>[6x]MAPKRKASSTCKTPKRQCIPKPGCCP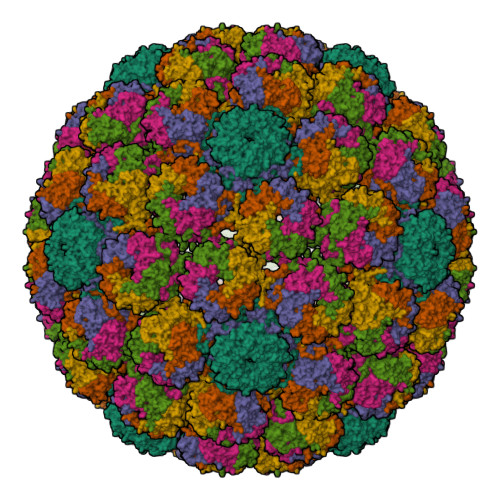NVASVPKLLVKGGVEVLSVVTGEDSITQIELYLNPRMGVNSPDLPTTSNWYTYTYDLQPKGSSPDQPIKENLPAYSVARVSLPMLNEDITCDTLQMWEAISVKTEVVGISSLINVHYWDMKRVHDYGAGIPVSGVNYHMFAIGGEPLDLQGLVLDYQTQYPKTTNGGPITIETVLGRKMTPKNQGLDPQAKAKLDKDGNYPIEVWCPDPSKNENSRYYGSIQTGSQTPTVLQFSNTLTTVLLDENGVGPLCKGDGLFISCADIVGFLFKTSGKMALHGLPRYFNVTLRKRWVKNPYPVVNLINSLFSNLMPKVSGQPMEGKDNQVEEVRIYEGSEQLPGDPDIVRFLDKFGQEKTVYPKPSVAPAAVTFQSNQQDKGKAPLKGPQKASQKESQTQEL(E)-4-((1-methylpiperidin-3-yloxyimino)methyl)benzimidamide | C14 H20 N4 O | 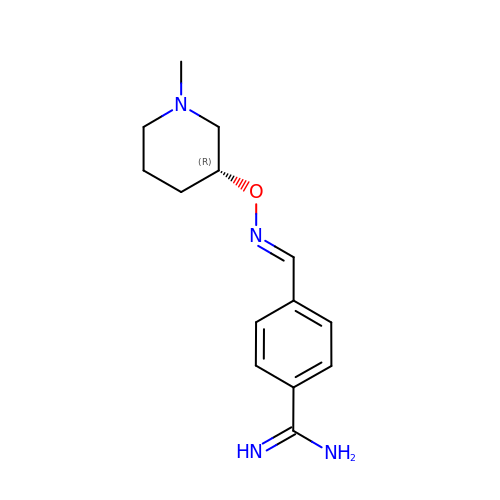GFIFKVKMSCQHRZ-LFMVTYOGSA-N To gain further insight into the structural conversions in pore formation, we chose pleurotolysin (Ply), a MACPF protein consisting of two components, PlyA and PlyB, from Pleurotus ostreatus. Previous studies have shown that PlyA binds membranes and is required to recruit the pore-forming MACPF protein PlyB to the membrane surface. PlyA and PlyB together form relatively small and regular pores in liposomes. The membrane attack complex/perforin-like family (MACPF) proteins form the largest superfamily of pore-forming proteins identified to date.

To probe the mechanism of pore assembly, we engineered a series of disulphide bonds to limit movement in either TMH1 or TMH2. As performed for perfringolysin O and other CDCs, the TMH regions were trapped by introducing cross-links to the central sheet or other adjacent regions in the monomer structure. This trapping allows oligomer assembly but prevents the TMH region from unfolding enough to insert into the membrane. The disulphide trap mutants were engineered on a background PlyB variant that lacks the wild type cysteine (C487A) in order to avoid incorrect disulphide bond formation. Oxidised TMH1 variant PlyBF138C,H221C (TMH1 lock) possessed no detectable lytic activity, but reduction of the disulphide restored wild type lytic activity. The crystal structure of the TMH1 trapped variant was determined and is otherwise indistinguishable from the wild type.

> MSQAGDTLNDVIQDPTRRNKLINDNNLLKGIIMGRDGPVPSSRELIVRPDTLRAIINNRATIETTTMEAEFTETLMESNYNSASVKVSAPCITANSEYSESSSFKNTETEKSMYTSSRYLFPQGRIDFTTPDSGFDDVIKLSPQFTSGVQAALAKATGTEKREALQNLFQEYGCVFRTKVHIGGVLSAHTMETFSRSENETEVKQDVKAGLEGAVKGWGGGATAGHGNTQGTITTSQNRKLNVKYIVNGGDYTKIQNTEEWVASTNQSEHWRVIEVTEVTAVADLLPQPIRGQVKDLLKPLLGKWVDVEKVPGLESLPVSVYRPKGAIPAGWFWLGDTADASKALLVKPTLPARSGRNPALTSLHQGSGMTEQPFVDLPQYQYLSTYFGSFAHDTPPGSTLRGLRPDHVLPGRYEMHGDTISTAVYVTRPVDVPFPEDEAFDLKSLVRVKLPGSGNPPKPRSALKKSMVLFDSGEK(2S,4S)-N-((3R,5R)-1-(cyclopropanecarbonyl)-5-((4-(((1R,2R)-2-(methoxymethyl)cyclopropyl)buta-1,3-diyn-1-yl)benzamido)methyl)pyrrolidin-3-yl)-4-fluoropyrrolidine-2-carboxamide | C30 H35 F N4 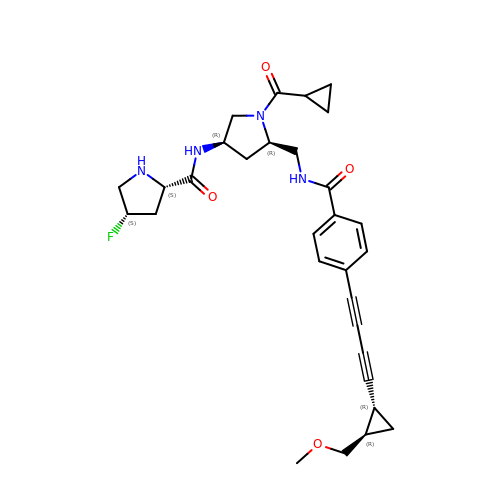O4 | WSHJZKFMSGXGDG-MSXPJASTSA-N>MENFTTNLNQLARVGGIDPLIGREKELERAIQVLCRRRKNNPLLVGESGVGKTAIAEGLAWRIVQGDVPEVMADCTIYSLDIGSLLAGTKYRGDFEKRFKALLKQLEQDTNSILFIDEIHTIIGAGAASGGQVDAANLIKPLLSSGKIRVIGSTTYQEFSNIFEKDRALARRFQKIDITEPSIEETVQIINGLKPKYEAHHDVRYTAKAVRAAVELAVKYINDRHLPDKAIDVIDEAGARARLMPVSKRKKTVNVADIESVVARIARIPEKSVSQSDRDTLKNLGDRLKMLVFGQDKAIEALTEAIKMARAGLGHEHKPVGSFLFAGPTGVGKTEVTVQLSKALGIELLRFDMSEYMERHTVSRLIGAPPGYVGFDQGGLLTDAVIKHPHAVLLLDEIEKAHPDVFNILLQVMDNGTLTDNNGRKADFRNVVLVMTTNAGVRETERKSIGLIHQDNSTDAMEEIKKIFTPEFRNRLDNIIWFDHLSTDVIHQVVDKFIVELQVQLDQKGVSLEVSQEARNWLAEKGYDRAMGARPMARVIQDNLKKPLANELLFGSLVDGGQVTVAL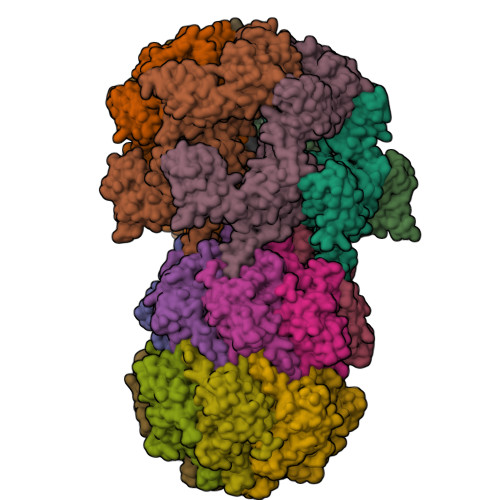DKEKNELTYGF[6x];>ALVPMVIEQTSRGERSFDIYSRLLKERVIFLTGQVEDHMANLIVAQMLFLEAENPEKDIYLYINSPGGVITAGMSIYDTMQFIKPDVSTICMGQAASMGAFLLTAGAKGKRFCLPNSRVMIHQPLGGYQGQATDIEIHAREILKVKGRMNELMALHTGQSLEQIERDTERDRFLSAPEAVEYGLVDSILTHR[14x]> NVAGINLLFKEGPKVNAKFELKPPPYPLNGLEPVMSQQTLEFHWGKHHRTYVENLKKQVVGTELDGKSLEEIIVTAYNKGDILPAFNNAAQVWNHDFFWECMKPGGGGKPSGELLELIERDFGSFEKFLDEFKAAAATQFGSGWAWLAYKASKLDGENAANPPSADEDNKLVVIKSPNAVNPLVWGGYYPLLTIDVWEHAYYLDFQNRRPDYISVFMDKLVSWDAVSSRLEQAKALS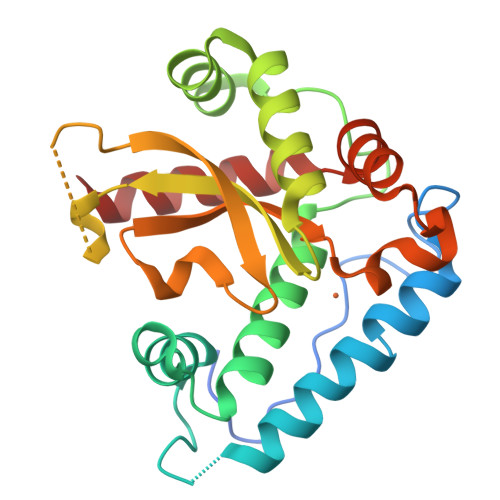A>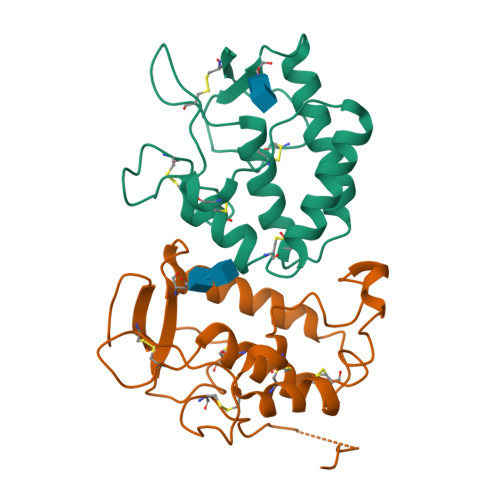[2x]ADLGSHHHHHHGPRGSKGYCAQYRGEVCDAVLVKDSLVFFNTSYPDPEEAQELLIHTAWNELKAVSPLCRPAAEALLCNHLFQECSPGVLPTPMPICREYCLAVKELFCAKEWLAMEGKTHRGLYRSGMHFLPVPECSKLPSMHQDPTACTRLPYLDYKKENITTFPSITSSKPSVDIPNLPASTSSFAVSPAYSMT Solution and crystal data are reported for DNA 18-mers with sequences related to those of bacterial noncoding single-stranded DNA segments called repetitive extragenic palindromes (REPs). REPs are DNA segments of about 30 nucleotides in length that occur frequently in some bacterial species. The center of the duplex is formed by two successive T–T mismatches.

In this study, we focus on two REP-related oligonucleotide sequences called Hpar-18 and Chom-18. The crystal structures of all three oligonucleotides, Chom-18, Chom-18Br and Hpar-18, were determined using highly anisotropic data at a relatively low resolution of worse than 2.6 Å. The subsequent refinement unequivocally established that all three 18-mers form antiparallel double helices in the crystal phase. The structures are highly similar: the calculated r.m.s.d. between all 365 non-H atoms of Chom-18 and Hpar-18 is 1.0 Å and the r.m.s.d. between Chom-18 and Chom-18Br is 0.24 Å. The crystal structures contain one central and one (in Hpar-18 and Chom-18Br) or two (in Chom-18) peripheral Sr2+ cations. In all three structures the central Sr2+ links the two O4 atoms of the symmetry-related mismatched thymines T9–T9*. In all cases the crystallization solutions contained Na+, a quadruplex-inducing metal, but also the quadruplex-breaking Mg2+ (in Chom-18 and Chom-18Br) and Li+ (in Hpar-18). In both the Chom-18 and Chom-18Br structures, all but two central steps are assigned to NtC classes, while in Hpar-18 two additional steps, 4–5 and 12–13, cannot be assigned and are formally assigned NtC class NANT. However, the unassigned steps are conformationally close to the A-like NtC classes, with a small r.m.s.d. from the closest NtC representatives of lower than 0.6 Å. The crystallographically unique TT di­nucleotides forming the mismatches, residues T9 and T10, are assigned to the frequently occurring NtC class AA08 in all three structures, with the preceding C8-T9 assigned to AA08 or AA00 and the following T10-G11 unassigned (NtC NANT).

> GGTGGGTCTTGACCCACC>LPNITILATGGTIAGGGDSATKSNYTAGKVGVENLVNAVPQLKDIANVKGEQVVNIGSQDMNDDVWLTLAKKINTDCDKTDGFVITHGTDTMEETAYFLDLTVKCDKPVVMVGAMRPSTSMSADGPFNLYNAVVTAADKASANRGVLVVMNDTVLDGRDVTKTNTTDVATFKSVNYGPLGYIHNGKIDYQRTPARKHTSDTPFDVSKLNELPKVGIVYNYANASDLPAKALVDAGYDGIVSAGVGNGNLYKTVFDTLAT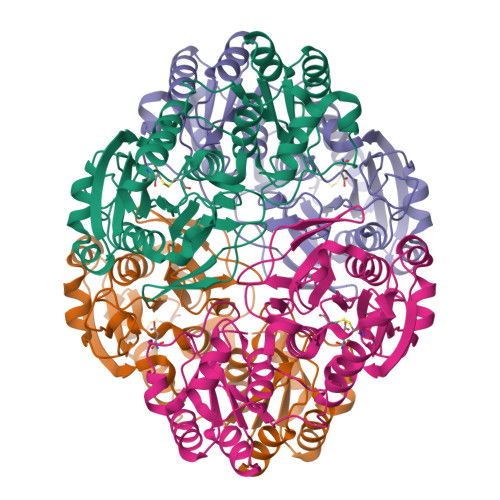AAKNGTAVVRSSRVPTGATTQDAEVDDAKYGFVASGTLNPQKARVLLQLALTQTKDPQQIQQIFNQY[2x]> QEIFQYVRLSQVKRDDK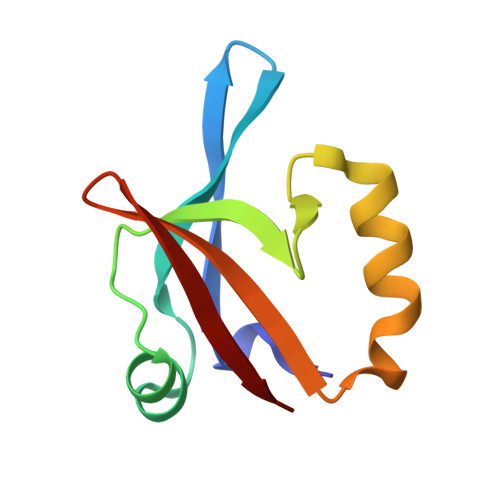VLGYRVSPGKDPVLFESIGLQDGDMAVALNGLDLTDPNVMNTLFQSMNEMTEMSLTVERDGQQHDVYIQF> MSFLFSSRSSKTFKPKKNIPEGSHQYELLKHAEATLGSGNLRQAVMLPEGEDLNEWIAVNTVDFFNQINMLYGTITEFCTEASCPVMSAGPRYEYHWADGTNIKKPIKCSAPKYIDYLMTWVQDQLDDETLFPSKI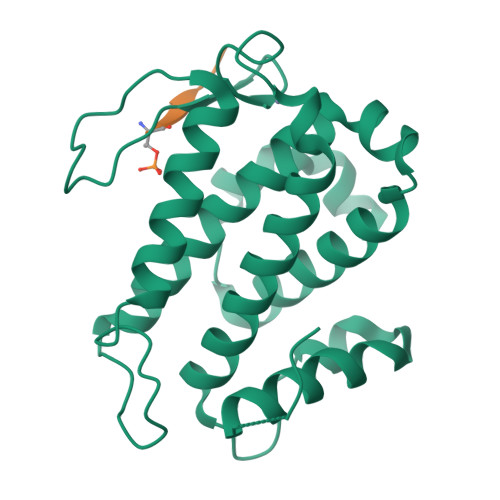GVPFPKNFMSVAKTILKRLFRVYAHIYHQHFDSVMQLQEEAHLNTSFKHFIFFVQEFNLIDRRELAPLQELIEKLGSKDR;> VASTMTDGANTMIEP> MTRQAYSSMLLSTAAALTLAFSLNASAAVDVDAA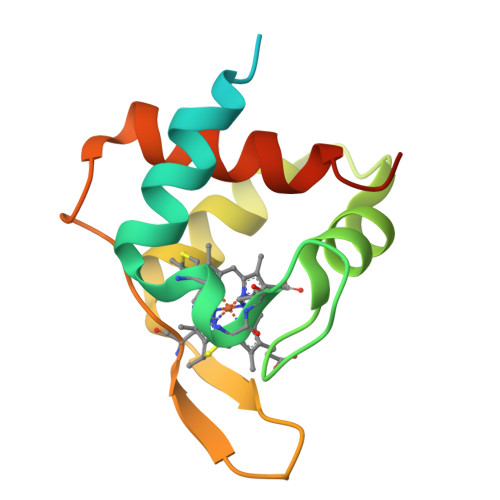KSLARENNCFKCHGVDKEKDGPSYKKVAEKYRGKADAEAKLIHHVTSGEKAKFPDGHEEEHKNINGKASPEAIKNLVDWILSLWSHPQFEK>MRSFLNLNSIPNVAAGNSCSIKLPIGQTYEVIDLRYSGVTPSQIKNVRVELDGRLLSTYKTLNDLILENTRHKRKIKAGVVSFHFVRPEMKGVNVTDLVQQRMFALGTVGLTTCEIKFDIDEAAAGPKLSAIAQKSVGTAPSWLTMRRNFFKQLNNGTTEIADLPRPVGYRIAAIHIKAAGVDAVEFQIDGTKWRDLLKKADNDYILEQYGKAVLDNTYTIDFMLEGDVYQSVLLDQMIQDLRLKIDSTMDEQAEIIVEYMG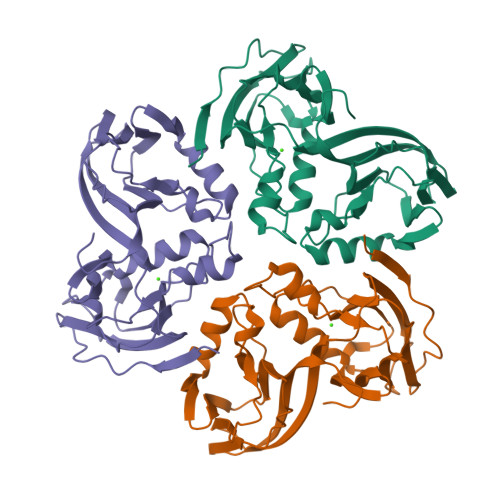VWSRNGF[6x]>[3x]QSTEASPKRSDGTPFPWNKIRLPEYVIPVHYDLLIHANLTTLTFWGTTKVEITASQPTSTIILHSHHLQISRATLRKGAGERLSEEPLQVLEHPRQEQIALLAPEPLLVGLPYTVVIHYAGNLSETFHGFYKSTYRTKEGELRILASTQFEPTAARMAFPCFDEPAFKASFSIKIRREPRHLAISNMPLVKSVTVAEGLIEDHFDVTVKMSTYLVAFIISDFESVSKITKSGVKVSVYAVPDKINQADYALDAAVTLLEFYEDYFSIPYPLPKQDLAAIPDFQSGAMENWGLTTYRESALLFDAEKSSASSKLDITMTVAHELAHQWFGNLVTMEWWNDLWLNEGFAKFMEFVSVSVTHPELKVGDYFFGKCFDAMEVDALNSSHPVSTPVENPAQIREMFDDVSYDKGACILNMLREYLSADAFKSGIVQYLQKHSYKNTKNEDLWDSMASICPTDGVKGMDGFCSRSQHSSSSSHWHQERVDVKTMMNTWTLQRGFPLITITVRGRNVHMKQEHYMKGSDGAPDTGYLWHVPLTFITSKSDMVHRFLLKTKTDVLILPEEVEWIKFNVGMNGYYIVHYEDDGWDSLTGLLKGTHTAVSSNDRASLINNAFQLVSIGKLSIEKALDLSLYLKHETEIMPVFQGLNELIPMYKLMEKRDMNEVETQFKAFLIRLLRDLIDKQTWTDEGSVSERMLRSELLLLACVHNYQPCVQRAEGYFRKWKESNGNLSLPVDVTLAVFAVGAQSTEGWDFLYSKYQFSLSSTEKSQIEFALCRTQNKEKLQWLLDESFKGDKIKTQEFPQILTLIGRNPVGYPLAWQFLRKNWNKLVQKFELGSSSIAHMVMGTTNQFSTRTRLEEVKGFFSSLKENGSQLRCVQQTIETIEENIGWMDKNFDKIRVWLQSEKLEHDPEADATGLERMLESRGPFEQKLISEEDLNMHTEHHHHHH;>XXTFPETLTY[3x]

The endoplasmic-reticulum aminopeptidase ERAP1 processes antigenic peptides for loading on MHC-I proteins and recognition by CD8 T cells as they survey the body for infection and malignancy. ERAP1 is a member of the M1 aminopeptidase family, which is found in all domains of life and plays numerous functional roles. These proteins contain a thermolysin-like domain10 (domain II), which holds the active site. The M1 aminopeptidase family has a conserved HEAT-motif-repeat domain (domain IV) forming a bowl-shaped C-terminal structure.

To begin to address how domain closure is coupled to catalysis, and to dissect structural features related to substrate binding from those related to the open-closed transition, we crystallized ERAP1 bound to the decamer phosphinic inhibitor, DG014, and determined the three-dimensional structure by X-ray crystallography DG014 shares DG013’s phosphinic group and N-terminal residues but is seven amino-acid residues longer, and similarly inhibits ERAP1 with high potency. Serendipitously, we were able to obtain crystals of the ERAP1–DG014 complex in the open conformer, and we determined its structure by X-ray crystallography (see “Methods” for details). The crystal structure shows that DG014 binds as expected with the phosphinic group at the active site, but with only the first five residues sufficiently structured to allow confident modeling. Ordered electron density of sufficient volume to contain ~2 amino-acid residues was observed 22 Å away from the active site, but we could not confidently ascertain whether this corresponded to buffer components or disconnected peptide C-terminal density, both of which have been observed at similar locations in domain IV in other crystal structures. A complex of ERAP1 bound to the long peptidomimetic inhibitor DG014 trapped crystallographically in the open conformation exhibited some of the conformational attributes previously observed in closed-state structures, in particular ordering of helix 4a, suggesting that these changes were coupled to substrate binding. Helix 4a is in an intermediate state in the open DG014 structure relative to closed-form structures, with a shift required to adopt the configuration present in the closed conformer. We suggest that the region between helices 4 and 5 (residues 426–433) acts as a sensor for substrate binding, ordering to form helix 4a in the presence of sufficiently long peptide-like substrates, and providing a site by which domain closure can be coupled to active-site reorganizations required for catalysis.> SMLNQFPGQYSNNIFCFPPIESETKSGKKASWIICVQVVQHNTIIPITDEMFSTDVKDAVAEIFTKFFVEEGAVRISKMTRVTEGKNLGKKNATTVVHQAFKDALSKYNRHARQKRGAHTNRGMIPPMLVKYFNIIPKTFFEEETDPIVQRKRN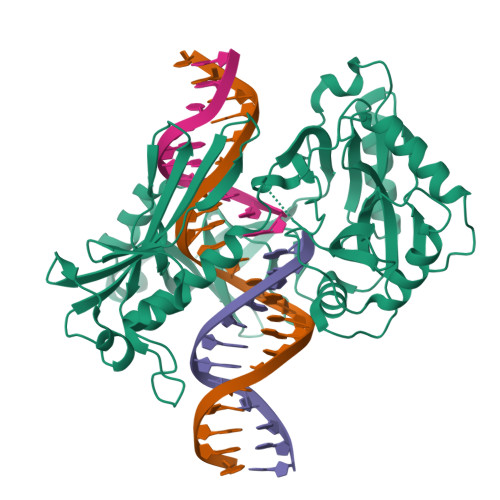GVRAVACQQGDGCILLYSRTEKEFLGLDNIKKELKQLYLFIDVRVYLDGELYLHRKPLQWIAGQANAKTDSSELHFYVFDCFWSDQLQMPSNKRQQLLTNIFKQKEDLTFIHQVENFSVKNVDEALRLKAQFIKEGYEGAIVRNANGPYEPGYNNYHSAHLAKLKPLLDAEFILVDYTQGKKGKDLGAILWVCELPNKKRFVVTPKHLTYADRYALFQKLTPALFKKHLYGKELTVEYAELSPKTGIPLQARAVGFREPINVLEII> MTSPQLEWTLQTLLEQLNEDELKSFKSLLWAFPLEDVLQKTPWSEVEEADGKKLAEILVNTSSENWIRNATVNILEEMNLTELCKMAKAEMMEDGQVQEIDNPELGDAEEDSELAKPGEKEGWRNSMEKQSLVWKNTFWQGDIDNFHDDVTLRNQRFIPFLNPRTPRKLTPYTVVLHGPAGVGKTTLAKKCMLDWTDCNLSPTLRYAFYLSCKELSRMGPCSFAELISKDWPELQDDIPSILAQAQRILFVVDGLDELKVPPGALIQDICGDWEKKKPVPVLLGSLLKRKMLPRAALLVTTRPRALRDLQLLAQQPIYVRVEGFLEEDRRAYFLRHFGDEDQAMRAFELMRSNAALFQLGSAPAVCWIVCTTLKLQMEKGEDPVPTCLTRTGLFLRFLCSRFPQGAQLRGALRTLSLLAAQGLWAQMSVFHREDLERLGVQESDLRLFLDGDILRQDRVSKGC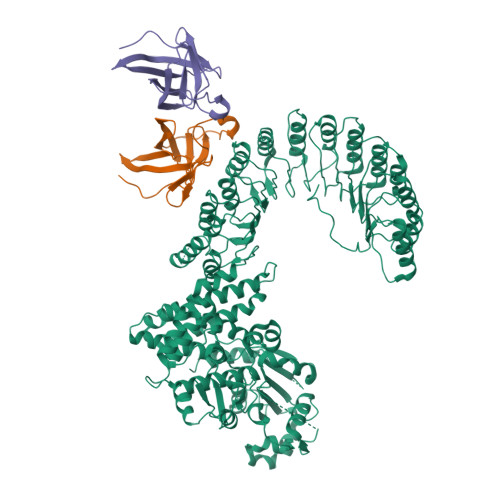YSFIHLSFQQFLTALFYALEKEEGEDRDGHAWDIGDVQKLLSGEERLKNPDLIQVGHFLFGLANEKRAKELEATFGCRMSPDIKQELLQCKAHLHANKPLSVTDLKEVLGCLYESQEEELAKVVVAPFKEISIHLTNTSEVMHCSFSLKHCQDLQKLSLQVAKGVFLENYMDFELDIEFERCTYLTIPNWARQDLRSLRLWTDFCSLFSSNSNLKFLEVKQSFLSDSSVRILCDHVTRSTCHLQKVEIKNVTPDTAYRDFCLAFIGKKTLTHLTLAGHIEWERTMMLMLCDLLRNHKCNLQYLRLGGHCATPEQWAEFFYVLKANQSLKHLRLSANVLLDEGAMLLYKTMTRPKHFLQMLSLENCRLTEASCKDLAAVLVVSKKLTHLCLAKNPIGDTGVKFLCEGLSYPDCKLQTLVLQQCSITKLGCRYLSEALQEACSLTNLDLSINQIARGLWILCQALENPNCNLKHLRLWSCSLMPFYCQHLGSALLSNQKLETLDLGQNHLWKSGIIKLFGVLRQRTGSLKILRLKTYETNLEIKKLLEEVKEKNPKLTIDCNASGATAPPCCDFFC;>EAVTDHPDRLWAWEKFVYLDEKQHAWLPLTIEIKDRLQLRVLLRREDVVLGRPMTPTQIGPSLLPIMWQLYPDGRYRSSDSSFWRLVYHIKIDGVEDMLLELLPDD[2x]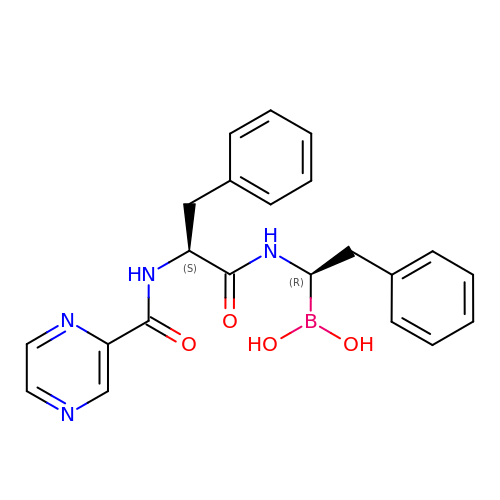N-[(1R)-1-(dihydroxyboranyl)-2-phenylethyl]-Nalpha-(pyrazin-2-ylcarbonyl)-L-phenylalaninamide | C22 H23 B N4 O4 | ILENEQWIGPQYCQ-ICSRJNTNSA-N>[2x]MKKILIVDDEKPISDIIKFNLAKEGYDTITAFDGREALSKYEEENPDLIILDLMLPELDGLEVAKEVRKNSHVPIIMLSAKDSEFDKVIGLEIGADDYVTKPFSNRELLARVKAHLRRTEN

VicR is a response regulator, which plays an important role in S. mutans growth and biofilm formation. Along with its cognate histidine kinase VicK, it constitutes the VicRK TCS that is involved in regulation of cell wall metabolism, nutrient uptake, osmotic protection, and biofilm formation. VicR possesses two domains, an N-terminal signal receiver domain and a C-terminal DNA binding domain. A typical TCS consists of a sensor histidine kinase and a response regulator, where the histidine kinase senses an environmental signal and relays the signal to a cognate response regulator, which in turn modulates expression of a cascade of effector genes.

To determine to which domain the 2-AI binds, recombinant N-terminal VicR (VicR-N) and C-terminal VicR (VicR-C) were generated and examined in the pulldown assay with the biotinylated 2-AI. Western blotting revealed that VicR-N and not VicR-C was captured by the biotinylated 2-AI (lanes 4 and 8), suggesting that the N terminus binds to this reverse amide 2-AI. To define the binding of VicR-N to 2B5, we attempted to solve the crystal structure of VicR-N in the presence of 2B5. We obtained diffractable crystals and determined the crystal structure of VicR-N using molecular replacement. VicR-N forms a dimer in the asymmetric unit. We also identified an unmodelled density surrounded by four negatively charged amino acids (Asp8, Asp9, Asp52, and Glu10) within the experimental structural map. To further investigate the binding, we docked 2B5 to VicR-N using AUTODOCK 4 and determined a binding energy of −4.98 kcal/mol. In the docking model, 2B5 is close to Asp9 (2.5 Å), Asp52 (2.6 Å), and Glu 10 (2.9 Å) of VicR-N, three of the negatively charged amino acids surrounding the undefined density shown in the experimental structure map. Further, we have demonstrated that the lead reverse amide 2-AI binds to the N-terminal signal receiver domain of VicR. This binding may inhibit the formation of the active VicR homodimer, which occurs at the N-terminal domain.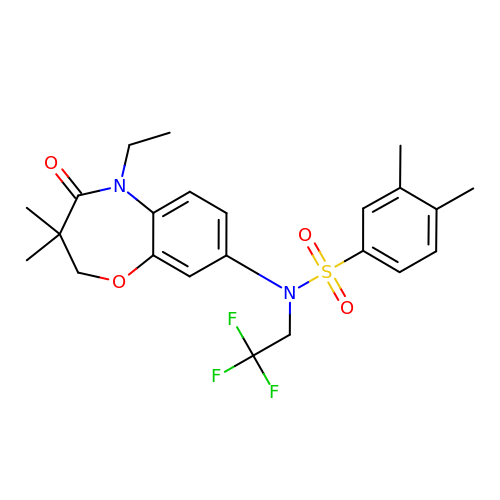N-(5-ethyl-3,3-dimethyl-4-oxo-2,3,4,5-tetrahydro-1,5-benzoxazepin-8-yl)-3,4-dimethyl-N-(2,2,2-trifluoroethyl)benzene-1-sulfonamide | C23 H27 F3 N2 O4 S | NWOKNZFZDJIXMB-UHFFFAOYSA-N>GHMRKLKIGITCYPSVGGSGIIATELGKQLAEKGHEIHFITSSIPFRLNTYHPNIHFHEVEVNQYAVFKYPPYDLTLASKIAEVAERENLDIIHAHYALPHAVCAYLAKQMLKRNIGIVTTLHGTDITVLGYDPSLKDLIRFAIESSDRVTAVSSALAAETYDLIKPEKKIETIYNFIDERVYLKKNTAAIKEKHGILPDEKVVIHVSNFRKVKRVQDVIRVFRNIAGKTKAKLLLVGDGPEKSTACELIRKYGLEDQVLMLGNQDRVEDLYSISDLKLLLSEKESFGLVLLEAMACGVPCIGTNIGGIPEVI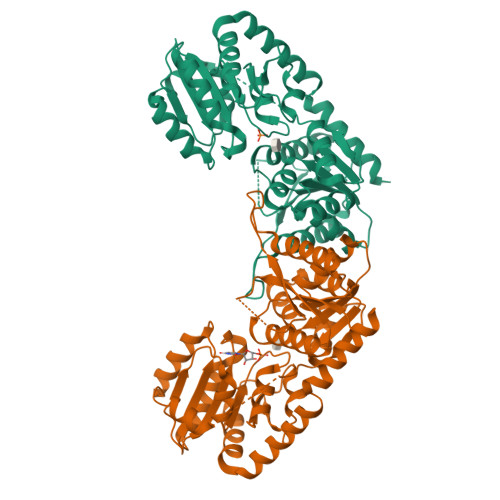KNNVSGFLVDVGDVTAATARAMSILEDEQLSNRFTKAAIEMLENEFSSKKIVSQYEQIYADLAEPE[2x]> FVNRGGLPVDEATWERMWKHVAKIHPDGEKVAQRIRGATDLPKIPIPSVPTFQPSTPVPERLEAVQRYIRELQYNHTGTQFFEIKKSRPLTGLMDLAKEMTKEALPIKCLEAVILGIYLTNSMPTLERFPISF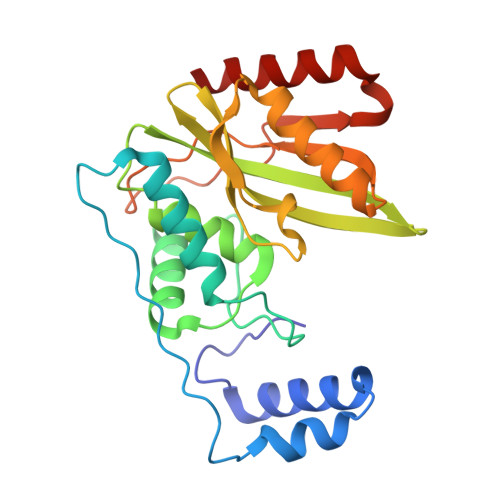KTYFSGNYFRHIVLGVNFAGRYGALGMSRREDLMYKPPAFRTLSELVLDFEAAYGRCWHVLKKVKLGQSVSHDPHSVEQIEWKHSVLDVERLGRDDFRKELERHARDMR>[2x]MDIWYGTAAVPKDLDNSAVTIGVFDGVH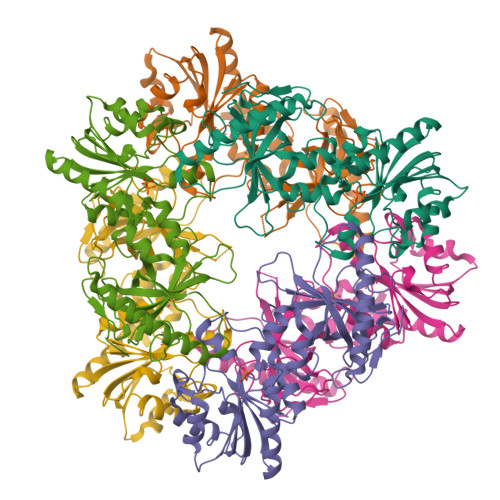RGHQKLINATVEKAREVGAKAIMVTFDPHPVSVFLPRRAPLGITTLAERFALAESFGIDGVLVIDFTRELSGTSPEKYVEFLLEDTLHASHVVVGANFTFGENAAGTADSLRQICQSRLTVDVIDLLDDEGVRISSTTVREFLSEGDVARANWALGRHFYVTGPVVRGAGRGGKELGFPTANQYFHDTVALPADGVYAGWLTILPTEAPVSGNMEPEVAYAAAISVGTNPTFGDEQRSVESFVLDRDADLYGHDVKVEFVDHVRAMEKFDSVAQLLEVMAKDVQKTRTLLAQDVQAHKMAPETYFLQAES>SIDVKYIG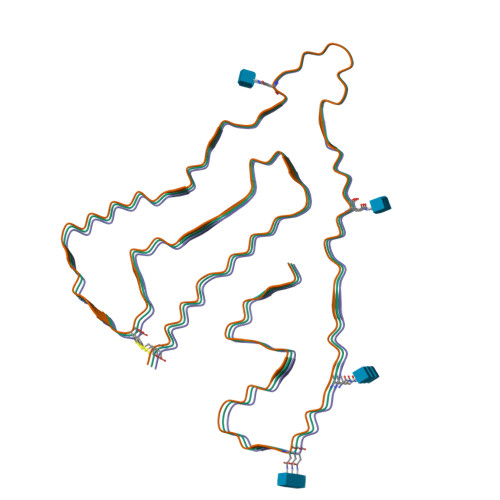VKSAYVSYDVQKRTIYLNITNTLNITNNNYYSVEVENITAQVQFSKTVIGKARLNNISIIGPLDMKQIDYTVPTVIAEEMSYMYDFCTLISIKVHNIVLMMQVTVTTTYFGHSEQISQERYQYVDCG[3x]>HHHHHHGSQQPTKTSNPNDQWTIKWSASDEFNKNDPDWAKWIKTGNLPNTSAWKWNNQKNVKISNGIAELTMRHNANNTPDGGTYFTSGIFKSYQKFTYGYFEAKIQGADIGEGVCPSFWLYSDFDYSVANGETVYSEIDVVELQQFDWYEGHQDDIYDMDLNLHAVVKENGQGVWKRPKMYPQEQLNKWRAPWDPSKDFHIYGCEVNQNEIIWYVDGVEVARKPNKYWHRPM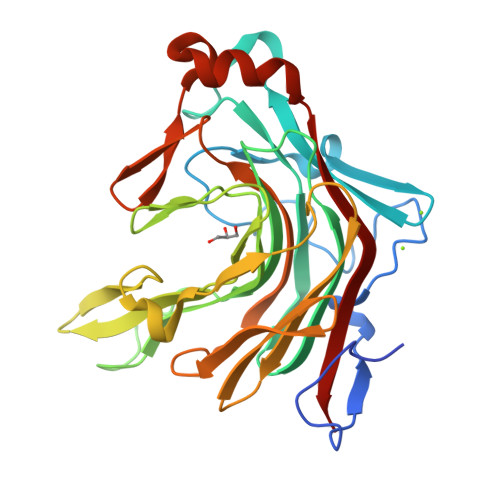NVTLSLGLRKPFVKFFDNKNNAINPETDAKAREKLSDIPTSMYVDYVRVWEKS[4x]>[2x]SKGQKLFVSVLQRLLSERGL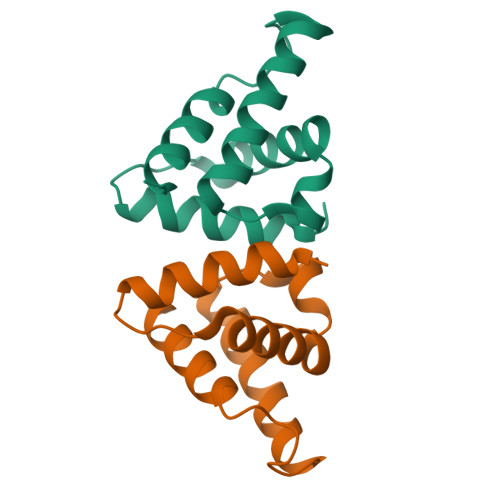HVKESSAIEFYQFLIKVSPWFPEEGGLNLQDWKRVGREMKRYAAEHGTDSIPKQAYPIWLQLREILT> NQSVVVDFLLPTGVYLNFPVSRNANLSTIKQLLWHRAQYE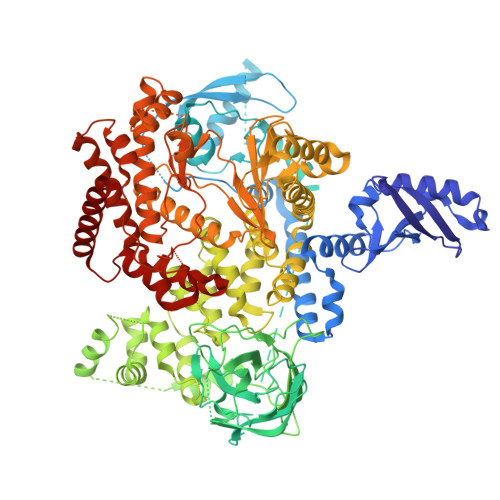PLFHMLSGPEAYVFTCINQTAEQQELEDEQRRLCDVQPFLPVLRLVAREGDRVKKLINSQISLLIGKGLHEFDSLCDPEVNDFRAKMCQFCEEAAARRQQLGWEAWLQYSFPLQLEPSAQTWGPGTLRLPNRALLVNVKFEGSEESFTFQVSTKDVPLALMACALRKKATVFRQPLVEQPEDYTLQVNGRHEYLYGSYPLCQFQYICSCLHSGLTPHLTMVHSSSILAMRDEQSNPAPQVQKPRAKPPPIPAKKPSSVSLWSLEQPFRIELIQGSKVNADERMKLVVQAGLFHGNEMLCKTVSSSEVSVCSEPVWKQRLEFDINICDLPRMARLCFALYAVIEKAKKARSTKKKSKKADCPIAWANLMLFDYKDQLKTGERCLYMWPSVPDEKGELLNPTGTVRSNPNTDSAAALLICLPEVAPHPVYYPALEKILELGRHSECVHVTEEEQLQLREILERRGSGELYEHEKDLVWKLRHEVQEHFPEALARLLLVTKWNKHEDVAQMLYLLCSWPELPVLSALELLDFSFPDCHVGSFAIKSLRKLTDDELFQYLLQLVQVLKYESYLDCELTKFLLDRALANRKIGHFLFWHLRSEMHVPSVALRFGLILEAYCRGSTHHMKVLMKQGEALSKLKALNDFVKLSSQKTPKPQTKELMHLCMRQEAYLEALSHLQSPLDPSTLLAEVCVEQCTFMDSKMKPLWIMYSNEEAGSGGSVGIIFKNGDDLRQDMLTLQMIQLMDVLWKQEGLDLRMTPYGCLPTGDRTGLIEVVLRSDTIANIQLNKSNMAATAAFNKDALLNWLKSKNPGEALDRAIEEFTLSCAGYCVATYVLGIGDRHSDNIMIRESGQLFHIDFGHFLGNFKTKFGINRERVPFILTYDFVHVIQQGKTNNSEKFERFRGYCERAYTILRRHGLLFLHLFALMRAAGLPELSCSKDIQYLKDSLALGKTEEEALKHFRVKFNEALRESWKT> MNNLHRELAPVSDAAWEQIEEEATRTLKRFLAARRVVDVTDPQGAALSAVGTGHVAYLDGPCAGVSAVKRQVLPVVEFRVPFKLTRQAIDDVERGSQDSDWSPLKEAARKIAAAEDQTIFDGYMAAGIAGIRPQSSNTPLTLPATASDYPTVVAQALDQLRV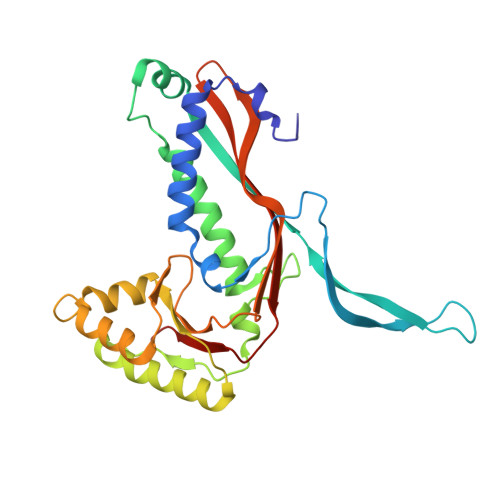AGVNGPYHLVLGEKAYTSITGGNEGGYPVFQHIRRLIDGEIVWAPAIEGGLLLTTRGGDFVMDIGQDISIGYLNHTGTDVELYLQESFTFSALTSEATVTLLPPEE> MGDQPFIPPPQQTALTVNDHDEVTVWNAAPCPMLPRDQVYVRVEAVAINPSDTKMRGQFATPWAFLGTDYAGTVVAVGSDVTHIQVGDRVYGAQNEMCPRTPDQGAFSQYTVTRGRVWAKIPKGLSFEQAAALPAGISTAGLAMKLLGLPLPSPSADQPPTHSKPV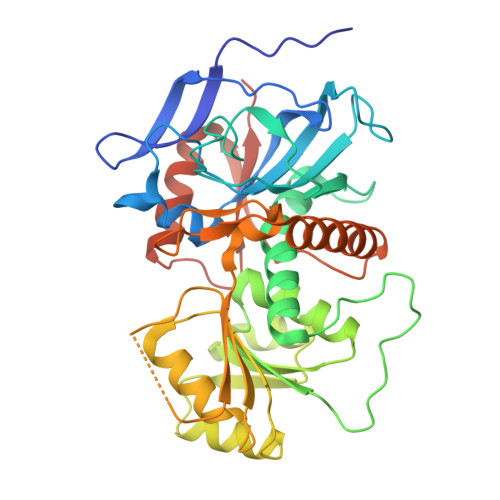YVLVYGGSTATATVTMQMLRLSGYIPIATCSPHNFDLAKSRGAEEVFDYRAPNLAQTIRTYTKNNLRYALDCITNVESTTFCFAAIGRAGGHYVSLNPFPEHAATRKMVTTDWTLGPTIFGEGSTWPAPYGRPGSEEERQFGEDLWRIAGQLVEDGRLVHHPLRVVQGGFDHIKQGMELVRKGELSGEKLVVRLEGPLEHHHHHH> MHHHHHHASAPALTKSQTDRLEVLLNPKDEISLNSGKPFRELESELLSRRKKDLQQIYAEERENYLGKLEREITRFFVDRGFLEIKSPILIPLEYIERMGIDNDTELSKQIFRVDKNFCLRPMLAPNLYNYLRKLDRALPDPIKIFEIGPCYRKESDGKEHLEEFTMLGFQQMGSGCTRENLESIITDFLNHLGIDFKIVGDSCMVYGDTLDVMHGDLELSSAGVGPIPLDREWGIDKPWIGAGFGLERLLKVKHDFKNIKRAARSESYYNGISTNL

We here report a novel, polyspecific Methanosarcina mazei PylRS mutant, DFRS2, capable of incorporating DFAs into proteins via ribosomal synthesis in vivo. Seeing that the poorly soluble PylRS N-terminal domain is not essential for amino acid activation, we employed a truncated form of DFRS2, DFRSc (residues 185-454), in our ATP-PPi exchange assays. We continued to determine the crystal structures of the DFRSc in complex with adenylyl-imidodiphosphate (AMP-PNP) and each of the six ncAAs 1-6 at 1.8–2.5 Å resolution. That is, D- and L-3-trifluoromethylphenylalanine (1 and 2); D- and L-3-chlorophenylalanine (3 and 4); and D- and L-3-bromophenylalanine (5 and 6).

Clear and well-defined electron density maps were also obtained from complexes between LFAs (2, 4, and 6) and DFRSc, exhibiting similar binding modes. We observed in the structures of LFA (2, 4, or 6)-bound DFRSc complexes that the carboxyl groups of LFAs form hydrogen bonds with residues L310 and A302 of DFRSc. As for DFRS2, we observed a significant increase in fluorescence in the presence of LFAs 2, 4, and 6, revealing amber stop codon suppression rates of 62.3%, 50.0% and 58.2%, respectively. Results indicated DFRS2 to display prominent aminoacylation activity with LFAs 2, 4, and 6, exhibiting K M of 0.09 ± 0.012, 0.05 ± 0.004, and 0.12 ± 0.010 mM, respectively. Our results revealed the K M of DFRSc to LFA 4 (5.38 ± 1.28 mM) to be lower than those to LFAs 2 (7.12 ± 1.67 mM) and 6 (9.80 ± 1.65 mM), whereas the k cat of DFRSc with LFAs 2, 4, and 6 (10.43 ± 0.37, 11.18 ± 0.29, and 10.21 ± 0.35 s-1 × 10−2, respectively) were similar. The relative aminoacylation efficiencies of DFRS2 with the ncAAs were then calculated based on the k cat/K M of PylRS with BocK, indicating the catalytic efficiency of DFRS2 with LFAs to be 1.2 to 2.3 folds higher, and contrastingly, those with DFAs to be 20 to 59 folds lower than PylRS with BocK.>CCAGATCT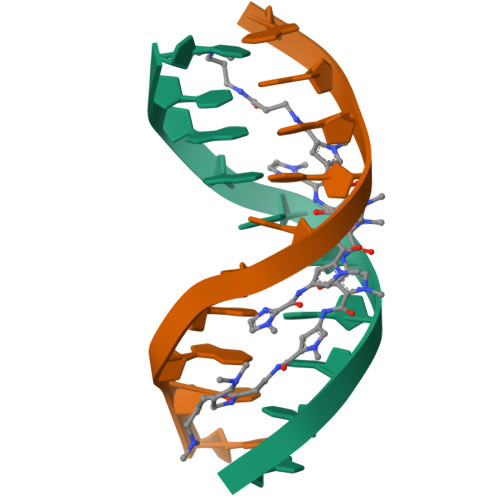GG[2x]>[2x]MSETPRLLFVHAHPDDESLSNGATIAHYTSRGAQVHVVTCTL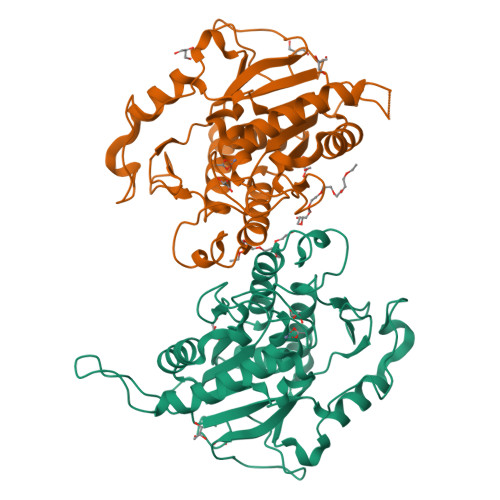GEEGEVIGDRWAQLTADHADQLGGYRIGELTAALRALGVSAPIYLGGAGRWRDSGMAGTDQRSQRRFVDADPRQTVGALVAIIRELRPHVVVTYDPNGGYGHPDHVHTHTVTTAAVAAAGVGSGTADHPGDPWTVPKFYWTVLGLSALISGARALVPDDLRPEWVLPRADEIAFGYSDDGIDAVVEADEQARAAKVAALAAHATQVVVGPTGRAAALSNNLALPILADEHYVLAGGSAGARDERGWETDLLAGLGFT> HHHHHHSQDPENLYFQGQEQAKVWTQTARANAEKNNAQLSTLLTDDQIGAIYGYTTNEGYTALNPALRGQTPLTPELEAFTGHVTDGLNKLPAYNGETYRGTTLPAHILEQNQIG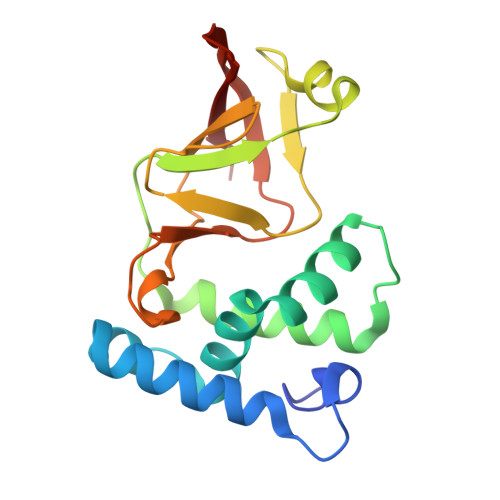GTVSDGGFMSTSAKTPFDGDVSISVRGNSGKQIDFLSKYKNEAEVLYPPNTRFEVINRIEQNGTTHLLYREIP> NLYFQHMRHFARTHAIGQIVA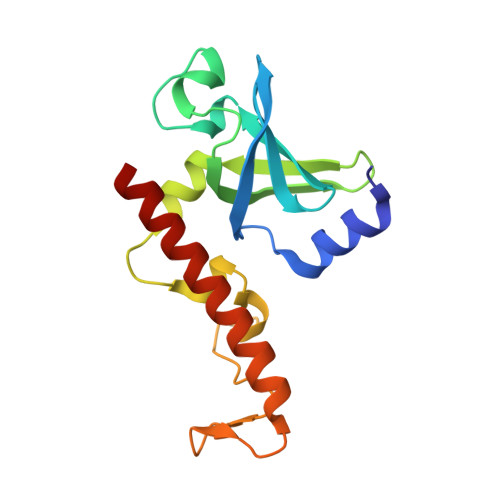GKVTKLVPFGAFVRVEEGIEGLVHISELAERHVEVPDQVVAVGDDAMVKVIDIDLERRRISLSLKQANEDYTEEFDPAKYGMADSYDEQGNYIFPEGFDAETNEWLEGFEKQRAEWEARYAEAERRHKMHTAQMEKF>[2x]MAN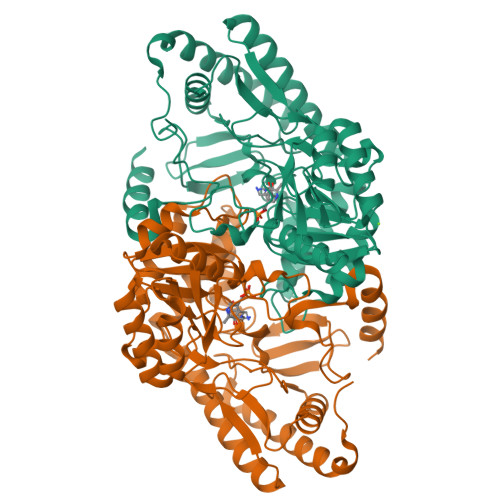GTRQKDLRERAERVIPGGMYGHESTRLLPPEFPQFFRRALGARIWDADEQPYIDYMCAYGPNLLGYRQSEIEAAADAQRLLGDTMTGPSEIMVNLAEAFVGMVRHADWAMFCKNGSDATSTAMVLARAHTGRKTILCAKGAYHGASPWNTPHTAGILASDRVHVAYYTYNDAQSLSDAFKAHDGDIAAVFATPFRHEVFEDQALAQLEFARTARKCCDETGALLVVDDVRAGFRVARDCSWTHLGIEPDLSCWGKCFANGYPISALLGSNKARDAARDIFVTGSFWFSAVPMAAAIETLRIIRETPYLETLIASGAALRAGLEAQSQRHGLELKQTGPAQMPQIFFADDPDFRIGYAWAAACLKGGVYVHPYHNMFLSAAHTVDDVTETLEATDRAFSAVLRDFASLQPHPILMQLAGAASSVDKLAAALEHHHHHH>[2x]KPVSL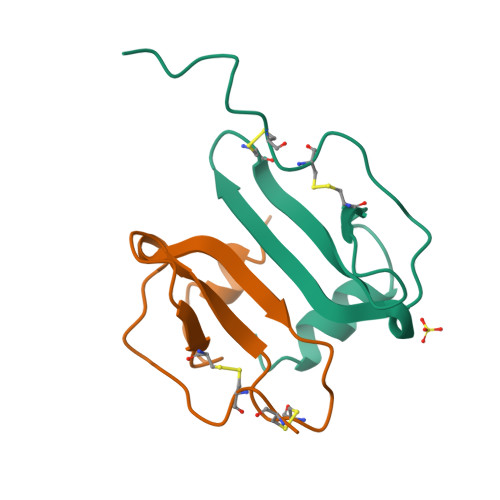SYRCPCRFFESHVARANVKHLKILNTPACALQIVARLKNNNRQVCIDPKLKWIQEYLEKALN Here we report the structure-function characterization of DC25, a protein from albumin fraction of Dolichos. The analysis resulted in identification of DC25, a 2S albumin homologue abundant in legumes. DC25 was characterized to be a monomeric thermostable protein. For the first time, we report DC25 being a plant origin oxidoreductase having peroxidase activity.

The structure of DC25 determined is at the highest resolution of 1.28 Å and provided better structural insights. The structure shows three monomers per asymmetric unit. Each monomer has a β-propeller domain, typical of the hemopexin superfamily proteins. The β-propeller domain is formed by circularly arranged four blades around the channel perpendicular to the plane of the blades. Each blade is composed of a β-sheet consisting of four antiparallel β-strands. The central channel consisted of four innermost β-strands of the blades, which are arranged in a parallel manner. The narrow end of the channel is lined with acidic amino acids, while the wider end is lined with basic amino acids. When the monomers of these proteins were superimposed, it was found that the core β-propeller structure was highly superimposable between DC25 and other three hemopexins from plant seeds with Cα RMSD values in the range of 0.32 Å to 0.54 Å. DC25, being homologous to CP4, LS24 and CAL, shows significant conformational differences in the loops connecting the outermost β-strands between the blades. Out of the 7 conserved water molecules, three water molecules (Wat428, 455, and 520) were present in the cavity whereas remaining four water molecules (Wat429, 437, 487 and 519) were buried and exist between the blade interfaces probably designed to stabilize the ß-propeller architecture.

>ASYINAAFRSSRAYEVYFFECNKYVRVYYTPGKTDDKILTNLRLISSGFPSLAGTAFAEPGIDCSFDTEASEAYVFSGSQCAYIDYAPGTTNDKILSGPTTIAEMFPVLKNTVFEDGIDSAFRSTKGKEVYLFKGNKYGRIAYDSKQLVGTIRNITDGFPVLKGTIFESGIDASFASHKEPEAYLFKGAQYVRIKFTPGATNNTLTGKVRPILDGWPCLRDILPT[3x]>MKLQVLPLSQEAFSAYGDVIETQQRDFFHINNGLVERYHDLALVEILEQDCTLISINRAQPANLPLTIHELERHPLGTQAFIPMKGEVFVVVVALGDDKPDLSTLRAFITNGEQGVNYHRNVWHHPLFAWQRVTDFL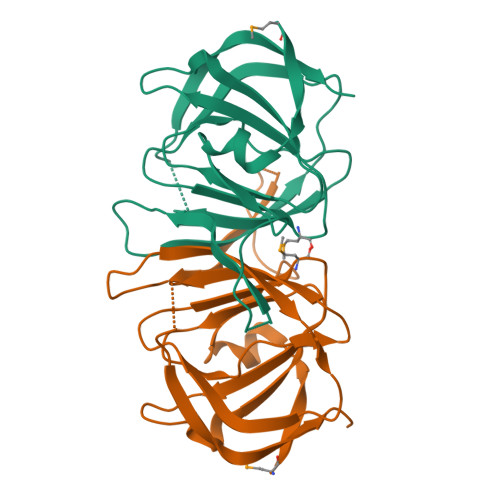TIDRGGSDNCDVESIPEQELCFALEHHHHHH[2x]>MGGGFAVNYNFDEIIDRRYTNAMNVEGYKGYLFGDADTSDLKDNDELIRMWVADMDFGTPEVVLNAIRERLNKKILGYTNVFGSEYYEAFVSWTKKRYGFTFSQEHLVFSHGIVAGLIELVGYICDKDDKALIVTPSYGPFKMACDKNHISTVYSPLINHHGYYEIDFDDVRKKVETENIKLCIFANPHNPTGRVWSEEELATLGQIMKENDVWLISDEIHCDIKRSGQSHIPFAKAVPDYDKIITTMSQSKAFNIAGLMFSNIIIQNESLLKTWNTHHFGTENPLSVVATQAAYEKGEGWLQAMNHYLDDNFNYLADFLEKELPHAEFKIPEATYLAWVDLSYYIKEKDIDESMAKFFIKNAGVIIEGAEQFVHNAEGHIRINIAVPREVMKKGLQKIKAALVENLYFQGHHHHHHHHHH[2x];> HHHHHH

Once inside the cell the terminal glycine is cleaved by a dipeptidase (PepA) to release Cys-3M3SH (2), which is metabolised by a C-S β-lyase liberating volatile 3M3SH (3), which diffuses or is exported out of the cell (4). While the PatB enzymes are poorly characterised and the genes are not associated with amino acid metabolism gene clusters or operons, the orthologues from B. subtilis (PatB) and Escherichia coli (MalY) are known to have cystathionine β-lyase activity, suggesting that these enzymes might also be capable of Cys-3M3SH cleavage. ShPatB and BsPatB are homodimeric with each subunit containing a PLP moiety covalently bound to a conserved lysine residue in the catalytic site (Lys246 and Lys234 in ShPatB and BsPatB, respectively) in what is termed the internal aldimine state. In the course of a typical PLP-DE catalysed reaction, upon substrate binding, the ε-amino group of the amino acid substrate displaces the lysine residue from the PLP to form an external aldimine.

In this study, we identify PatB in S. hominis as the C-S lyase responsible for thioalcohol liberation from Cys-3M3SH. In particular, ShPatB exhibits selectivity towards Cys-3M3SH with a catalytic efficiency 138-fold higher that that towards cystathionine (766 M−1 min−1 and 5.53 M−1 min−1, respectively). Absorption spectra indicate the presence of PLP (410 nm) covalently bound to ShPatB. ShPatB is a PLP-DE, with a core active site that is structurally conserved across all C-S lyases; however, ShPatB contains a hydrophobic pocket comprising unique residues not found in any other PatB enzymes other than malodour producing staphylococci. This hydrophobic pocket in ShPatB is essential for Cys-3M3SH selectivity. The introduction of a Tyr25Ala substitution resulted in a sixfold increase in KM, significantly affecting Cys-3M3SH binding compared to wild-type ShPatB. The shape of the hydrophobic pocket is critical for Cys-3M3SH binding; mutating Thr276 to Ala resulted in an 8.5-fold increase in ShPatB KM for Cys-3M3SH. ShPatB clearly prefers branched aliphatic side chains followed by linear hydrophobic side groups while excluding linear charged ligands. In contrast to the roles of other MalY-type PatB enzymes as redundant MetC replacements in sulphur-containing amino acid metabolism, ShPatB is selective for aliphatic cysteine-S-conjugates only, while discriminating against polar ligands such as cystathionine.> MKDFLRLELPVLPLRNTVVLPHTTTGVDVGRLKSKRAVEEALSADRLLFLVTQKDPEVDDPAPEDLYAVGTLAVVKQAMRLPDGTLQVMVEARSRARLLSYVAAPYLRAVGEAIPEPPLKDPEL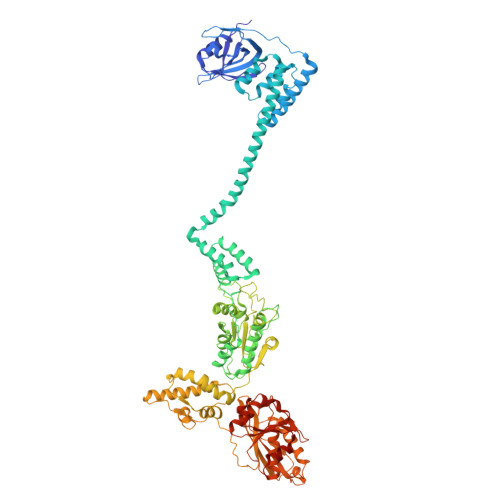ARVLVNEVQEAFERYLQNHKTLRLDRYQQEAVKSTRDPAILADLVAHHATWTLEEKQTILETPEVEERLKRVLALLLRDLERFELDKKIAARVKEQMDQNQREYYLREQMKAIQKELGGGEDFLTEIEELRERIEKKGMPEPVKEKALKELKRLERMQPGSPEATVSRTYLDWLLEVPWTEADPEVLDISVTKRVLDEDHYGLKEVKERILEYLAVRQLTQGKEVKGHAPILCFVGPPGVGKTSLGKSIARSMNRRFHRISLGGVRDEAEIRGHRRTYIGALPGKIIQGMKQVGVVNPVFLLDEIDKLSSDWRGDPAAALLEVLDPEQNHTFTDHYLDVPYDLSKVFFITTANTLSTIPRPLLDRMEVIEIPGYTLHEKRAIARYFRWPFQVKEAGLEGRLEITDRAIERIVQEYTREAGVRNLDRELSKVARKAAKDYLEKPWEGVRVVDAEDLEAYLGVPKYRPDRAEKEPQVGAAQGLAWTPYGGTLLTIEAVAVPGTGKVNLTGNLGEVMKESAHAALTYLRAHREEWGLPEGFHKDYDLHIHVPEGATPKDGPSAGITIATALASALTGRPVRMDIAMTGEITLRGRVLPIGGVKEKLLAAHQAGIHRVILPKENAAELKEVPEEILKDLEIHFVEEVGEVLKLLLLPPPPPPAVQPDRPQPGVGA> VYTSTETSHIDQESYNFFEKYARLANIGYCVGPGTKIFKPFNCGLQCAHFPNVELIEEFHDPRLIFDVSGYLAVDHASKQIYLVIRGTHSLEDVITDIRIMQAPLTNFDLAAQISSTATCDDCLVHNGFIQSYQNTYNQIGPKLDSVIEQYPDYQIAVTGHSLGGAAALLFGINLKVNGHDPLVVTLGQPIVGNAGFANWVDKLFFGQENPDVSKVSKDRKLYRITHRGDIVPQVPFWDGYQHCSGEVFIDWPLIHPPLSNVVMCQGQSNKQCSAGNTLLQQVNVIGNHLQYF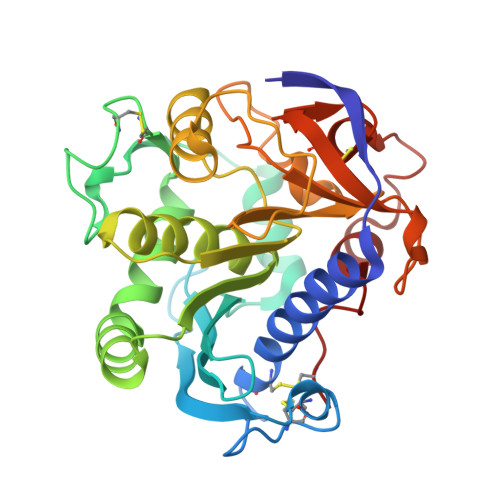VTEGVCGI>[48x]MNNLYRDLAPVTEAAWAEIELEAARTFKRHIAGRRVVDVSDPGGPVTAAVSTGRLIDVKAPTNGVIAHLRASKPLVRLRVPFTLSRNE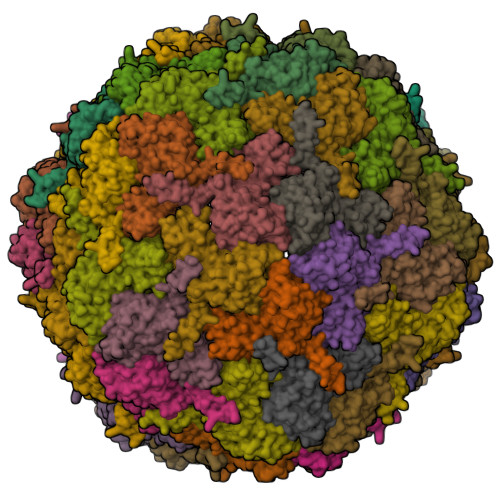IDDVERGSKDSDWEPVKEAAKKLAFVEDRTIFEGYSAASIEGIRSASSNPALTLPEDPREIPDVISQALSELRLAGVDGPYSVLLSADVYTKVSETSDHGYPIREHLNRLVDGDIIWAPAIDGAFVLTTRGGDFDLQLGTDVAIGYASHDTDTVRLYLQETLTFLCYTAEASVALSH5'-{[(3S)-3-amino-3-carboxypropyl]({1-[(4-chlorophenyl)methyl]azetidin-3-yl}methyl)amino}-5'-deoxyadenosine 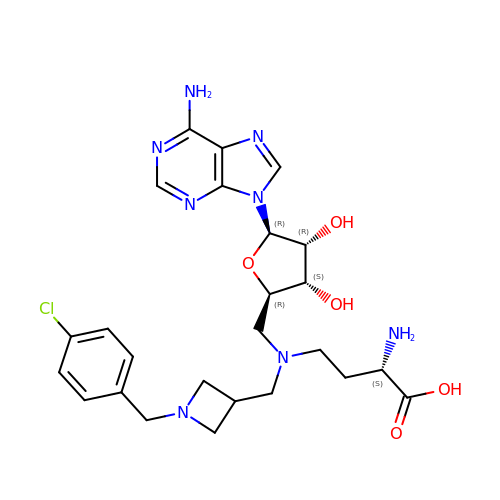| C25 H33 Cl N8 O5 | BNFSVXBSRYHZTB-XCPBYIKRSA-N Collagen prolyl 4‐hydroxylase (C‐P4H) catalyzes the 4‐hydroxylation of Y‐prolines of the XYG‐repeat of procollagen. The α‐subunit provides the N‐terminal dimerization domain, the middle peptide‐substrate–binding (PSB) domain, and the C‐terminal catalytic (CAT) domain. There are three isoforms of the α‐subunit, complexed with a β‐subunit that is protein disulfide isomerase, forming C‐P4H I‐III. The PSB domain of the α‐subunit binds proline‐rich peptides, but its function with respect to the prolyl hydroxylation mechanism is unknown.

An extended mode of binding of proline‐rich peptides (PPII, polyproline type‐II, conformation) to the PSB‐I domain has previously been reported for the PPG‐PPG‐PPG and P9 peptides. Crystal structures now show that peptides with the motif PxGP (PPG‐PRG‐PPG, PPG‐PAG‐PPG) (where x, at Y‐position 5, is not a proline) bind to the PSB‐I domain differently, more deeply, in the peptide‐binding groove. The latter mode of binding has previously been reported for structures of the PSB‐II domain complexed with these PxGP‐peptides. Calorimetric binding studies show that the affinities of these peptides are lower for PSB‐I than for PSB‐II, with, respectively, K D values of about 70 μM for PSB‐I and 20 μM for PSB‐II.

>[4x]MSFLTAEDCFELGKVAYTEADYYHTELWMEQALRQLDEGEISTIDKVSVLDYLSYAVYQQGDLDKALLLTKKLLELDPEHQRANGNLKYFEYIMAKELEHHHHHH;>PPGPRGPPG[3x]> QTIQSIPQKGFFGHPRGLGVLFFVEFWERFSYYGMRAMLIFYMYFAIHQNGLGIDKTTAMSIMSVYGALIYMSSIPGAWIADRITGTRGATLLGAVLIIIGHICLSLPFALFGLFSSMFFIIIGSGLMKPNISNIVGRLYPENDTRIDAGFVIFYMSVNLGALISPIILQHFVDIRNFHGGFLLAAIGMALGLVWYLLFNRKNLGSVGMKPTNPLSKEEKRKYGMIIGIIVAIVIVVLLVTYYTHTLSFDLISNTVLVLGVALPIIYFTTMLRSKDVTDGERSRVKAFIPLFILGMLFWSIQEQGSNVLNIYGLERSDMQLNLFGWTTRFGEALFQSINPLFILLFAPVISMIWLKMGKKQPSL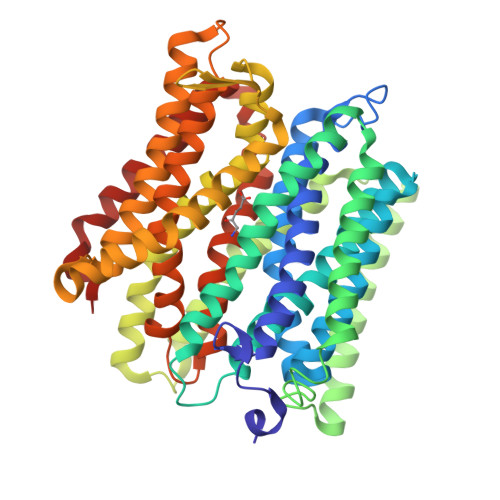AIKFSIGTLLAGLSYILIGLVGLGYGHTQFSVNWVILSYVICVIGELCLSPTGNSAAVKLAPKAFNAQMMSVWLLTNASAQAINGTLVKLIKPLGQTNYFIFLGTVAIVITLIILVFSPKITK> SNAVDLSDADTLQRYLDQRFQQVDVSVKLELWHEAYRSIEDVFHLMKISKRAPKPSTLANYYENLVKVFFVSGDPLLHTTAWKKFYKLYSTNPRATEEEFKTYSSTIFLSAISTQLDEIPSIGYDPHLRMYRLLNLDAKPTRKEMLQSIIEDESIYGKVDEELKELYDIIEVNFDVDTVKQQLENLLVKLSSKTYFSQYIAPLRDVIMRRVFVAASQKFTTVSQSELYKLATLPAPLDLSAWDIEKSLLQAAVEDYVSITIDHESAKVTFAKDP;> MDQAVQEDFFTRLQTIIDSRGKKTVNQQSLISTLEELLTVAEKPYEFIMAYLTLIPSRFDASANLSYQPIDQWKSSFNDISKLLSILDQTIDTYQVNEFADPIDFIEDEPKEDSDGVKRILGSIFSFVERLDDEFMKSLLNIDPHSSDYLIRLRDEQSIYNLILRTQLYFEATLKDEHDLERALTRPFVKRLDHIYYKSENLIKIMETAAWNIIPAQFKSKFTSKDQLDSADYVDNLIDGLSTILSKQNNIAVQKRAILYNIYYTALNKDFQTAKDMLLTSQVQTNINQFDSSLQILFNRVVVQLGLSAFKLCLIEECHQILNDLLSSSHLREILGQQSLHRISLNSSNNASADERARQCLPYHQHINLDLIDVVFLTCSLLIEIPRMTAFYSGIKVKRIPYSPKSIRRSLEHYDKLSFQGPPETLRDYVLFAAKSMQKGNWRDSVKYLREIKSWALLPNMETVLNSLTERVQVESLKTYFFSFKRFYSSFSVAKLAELFDLPENKVVEVLQSVIAELEIPAKLNDEKTIFVVEKGDEITKLEEAMVKLNKEYKIAKERLNPPSNRR

Eukaryotic translation initiation requires the recruitment of the large, multiprotein eIF3 complex to the 40S ribosomal subunit. EIF3 is a large and structurally complex molecular assembly that, in the majority of eukaryotes, consists of 11–13 subunits (eIF3a-eIF3m) with a molecular weight of 600–800 kDa. We present X-ray structures of all major components of the minimal, six-subunit Saccharomyces cerevisiae eIF3 core. Yeast eIF3 engages 40S in a clamp-like manner, fully encircling 40S to position key initiation factors on opposite ends of the mRNA channel, providing a platform for the recruitment, assembly, and regulation of the translation initiation machinery.

Using the full eIF3a PCI-domain structure as a guide, N-terminal eIF3a truncations were generated to obtain crystals of a dimeric eIF3a/eIF3c assembly, encompassing the full predicted PCI domain of eIF3c (S. cer. residues 251–812) and residues 228–496 of eIF3a. The structure of the dimeric eIF3a/eIF3c complex was solved at 3.5 Å resolution using Se-Met SAD. As expected, the PCI domain of eIF3c shares the basic architecture of the fold but with a more elaborate helical domain that extends over 450 residues. The helical domain can be subdivided into two regions: helical-element 1 (HE-1) is composed of helices 1–7, whereas helical element 2 (HE-2) contains helices 9–13. HE-1 and HE-2 form TPR-like right-handed superhelices similar to those found in other PCI proteins, with the relative orientations of HE-1 and HE-2 defined by helix 8, which disrupts the helical repeat at the HE-1/HE-2 interface, inducing an almost 90° bend in the domain. An extensive, conserved protein segment formed by a 40 amino acid insertion between helices 13 and 17 meanders back into the HE-1/HE-2 interface to further stabilize the kink. The dimerization interface between eIF3a and eIF3c involves two distinct interaction regions. Helix 23 in the WHD of eIF3a engages the WHD of eIF3c in an arrangement similar to the Thp1-Sac3 PCI-dimer (Ellisdon et al., 2012). The second interaction interface between eIF3a and eIF3c involves a loop between helices 18 and 19 of eIF3c that engages a cleft formed by helices 11, 12, and 15 of eIF3a, allowing a stacking interaction between residue F664 of eIF3c and Y257 of eIF3a. This interaction induces a rearrangement of up to 3 Å at the end of eIF3a helix 15 to accommodate the eIF3c loop.>[2x]GDDLEVGKNIDESAYSGIYENNAYLRDGKSNLVSKVVELHGETYATTVKMGLSKTPNTATSAKVKIDAAYLETYNKAHNTDFALYPQDLVTFANEGILTVNANTKSAEVEMTIRAGEGLQEDKTYAIPVAISDQSSDITIKDEDAKHCIYLVKDMRNAGDAYKGEGVMQGYLFFEVNDVNPLNTLSFQLENGKLLWDVVVLFAANINYDAEAGRPRVQCNPNVQYLLDNNETLLQPLRRRGVKVLLGLLGNHDITGLAQLSEQGAKDFAREVAQYCKAYNLDGVNYDDEYSNSPDLSNPSLTNPSTAAAARLCYETKQAMPDKLVTVFDWGQMYGVATVDGVDAKEWIDIVVANYGSAAYPIGQMTKKQCSGISMEFNLGGGGSLSASKAQSMIDGGYGWFMGFAPSPAKYGSVFSRLQGGGEVLYGSNVAAPTIFYKKNDPTPYKYPDDL

EndoBT-3987 is a secreted enzyme that initiates the HM degradation pathway and hydrolyzes the oligosaccharide from its polypeptide chain on the cell surface. ENGases are endoglycosidases that hydrolyze the chitobiose core of N-linked glycans (EC 3.2.1.96). Residues 26–41 were not visible in the structure. The full-length EndoBT-3987 comprises two domains from the N- to the C-terminus: (i) a β-sandwich domain (42–179) followed by a short linker (residues 180–193) that continues to (ii) a GH domain (residues 194–476). Here, we provide the high-resolution X-ray crystal structures of EndoBT-3987 in its unliganded form, in complex with its substrate, Man9GlcNAc2Asn, and two of its products, Man5GlcNAc and Man9GlcNAc.

The strategy for capturing a native binary enzyme-product complex was to perform co-crystallization experiments with the full-length EndoBT-3987 (EndoBT-3987WT) in the presence of Man5GlcNAc2Asn or Man9GlcNAc2Asn substrates. Two crystal forms were obtained for the EndoBT-3987WT-GlcNAcMan9 complex, in space groups P1 (EndoBT-3987WT-Man9GlcNAc-1) and P 21 21 21 (EndoBT-3987WT-Man9GlcNAc-2), and the corresponding crystal structures solved at 2.0 and 1.7 Å resolution, respectively. The overall protein scaffold and the conformation of the EndoBT-3987WT-Man5GlcNAc (r.m.s.d. of 0.35 Å for 397 residues), EndoBT-3987WT-Man9GlcNAc-1 (r.m.s.d. of 0.48 Å for 397 residues) and EndoBT-3987WT-Man9GlcNAc-1 (r.m.s.d. of 0.41 Å for 397 residues) crystal structures were essentially preserved with respect to the EndoBT-3987D312A/E314L-Man9GlcNAc2Asn substrate complex.> MRSALRLA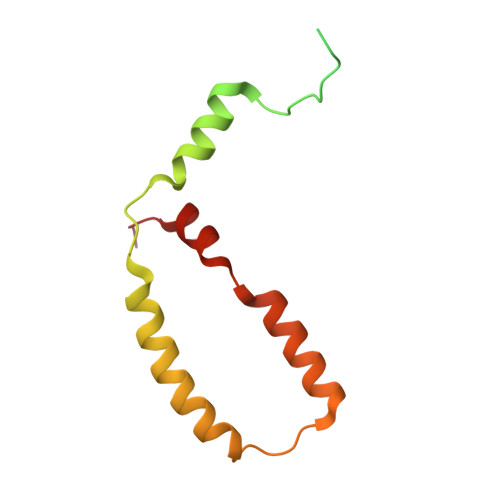NATRLSTFRLTSAPAVRLASPSFFVQKEDEENTRSIHTSNSSFHDEPKHQIPGNALDNWAFLRTYAKPLPDMIHYYYYVYLFGFFFVYKVADFPEYSPRVLVMAALIGSLFYVRRDWVHREFKDSP> MSLSQRTLLLLSQDNAHYERLLKAAHLPHLRILRADNQSDAEKLIGEAHILMAEPARAKPLLAKANKLSWFQSTYAGVDVLLDARCRRDYQLTNVRGIFGPLMSEYVFGHLLSLMRQLPLYREQQKQRLWQSHPYQGL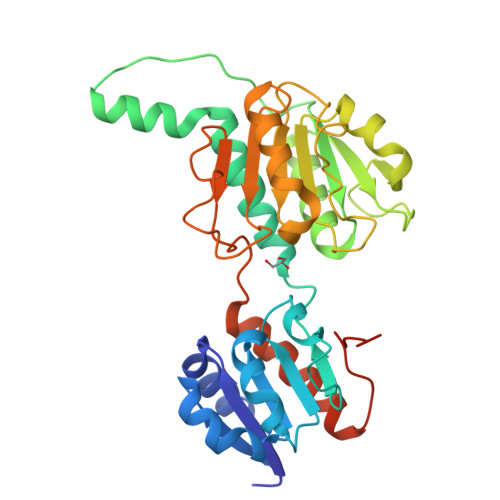KGRTLLILGTGSIGQHIAHTGKHFGMKVLGVSRSGRERAGFDQVYQLPALNKMLAQADVIVSVLPATRETHHLFTASRFEHCKPGAILFNVGRGNAINEGDLLTALRTGKLGMAVLDVFEQEPLPADSPLWGQPNLIITPHNSAYSFPDDVAQIFVRNYIRFIDGQPLDGKIDFDKGYEGHHHHHH> MSEFNITETYLRFLEEDTEMTMPIAAIEALVTLLRIKTPETAAEMINTIKSSTEELIKSIPNSVSLRAGCDIFMRFVLRNLHLYGDWENCKQHLIENGQLFVSRAKKSRNKIAEIGVDFIADDDIILVHGYSRAVFSLLNHAANKFIRFRCVVTESRPSKQGNQLYTLLEQKGIPVTLIVDSAVGAVIDKVDKVFVGAEGVAESGGIINLVGTYSVGVLAHNARKPFYVVTESHKFVRMFP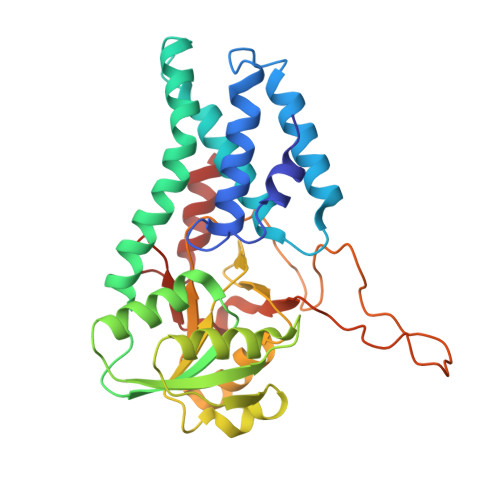LSSDDLPMAGPPLDFTRRTDDLEDALRGPTIDYTAQEYITALITDLGVLTPSAVSEELIKMWYD>[2x]MHEWALADAIVRTVLDYAQREGASRVKAVRVVLGELQDVAEDIVKFAMEQLFAGTIAEGAEIEFVEEEAVFKCRNCNYEWKLKEVKDKFDERIKEDI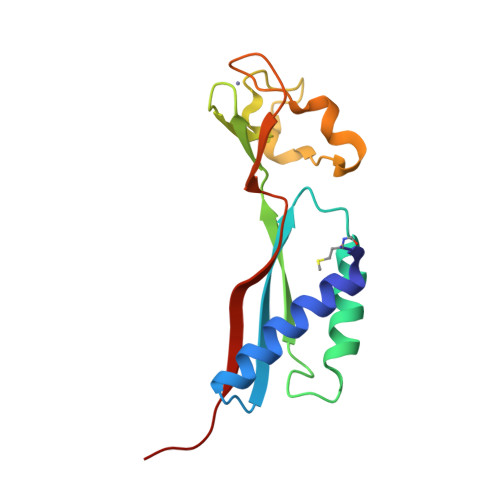HFIPEVVHAFLACPKCGSHDFEVVKGRGVYVAGIKIEKEGGS> GSGSGTPAPPAIADLLASVDSEEVRDYCRTKG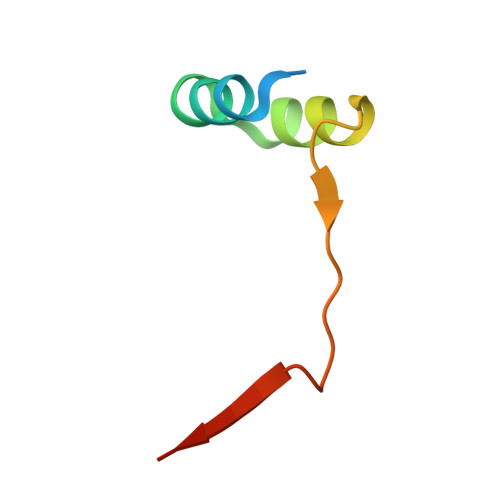WIVQEKITKESLERNVNR> MSYYHHHHHHSSGENLYFQGHKYKKQFRYESQLQMVQVTGSSDNEYFYVDFREYEYDLKWEFPRENLEFGKVLGSGAFGKVMNATAYGISKTGVSIQVAVKMLKEKADSSEREALMSELKMMTQLGSHENIVNLLGACTLSGPIYLIFEYCCYGDLLNYLRSKREKFHRTWTEIFKEHNFSFYPTFQSHPNSSMPGSREVQIHPDSDQISGLHGNSFHSEDEIEYENQKR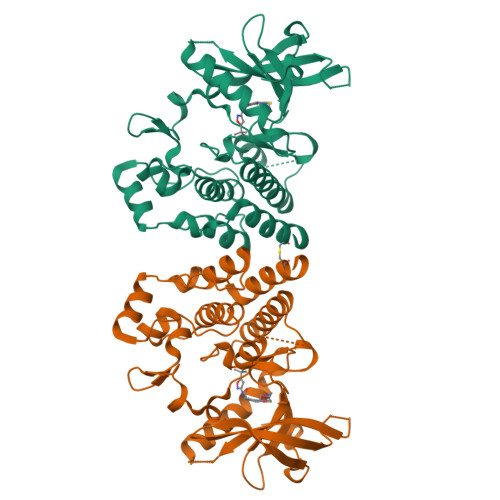LEEEEDLNVLTFEDLLCFAYQVAKGMEFLEFKSCVHRDLAARNVLVTHGKVVKICDFGLARDIMSDSNYVVRGNARLPVKWMAPESLFEGIYTIKSDVWSYGILLWEIFSLGVNPYPGIPVDANFYKLIQNGFKMDQPFYATEEIYIIMQSCWAFDSRKRPSFPNLTSFLGCQLADAEEAMYQNV> MSADSSPLVGSTPTGYGTLTIGTSIDPLSSSVSSVRLSGYCGSPWRVIGYHVVVWMMAGIPLLLFRWKPLWGVRLRLRPCNLAHAETLVIEIRDKEDSSWQLFTVQVQTEAIGEGSLEPSPQSQAEDGRSQAAVGAVPEGAWKDTAQLHKSEEAVSVGQKRVLRYYLFQGQRYIWIETQQAFYQVSLLDHGRSCDDVHRSRHGLSLQDQMVRKAIYGPNVISIPVKSYPQLLVDEALNPYYGFQAFSIALWLADHYYWYALCIFLISSISICLSLYKTRKQSQTLRDMVKLSMRVCVCRPGGEEEWVDSSELVPGDCLVLPQEGGLMPCDAALVAGECMVNESSLTGESIPVLKTALPEGLGPYCAETHRRHTLFC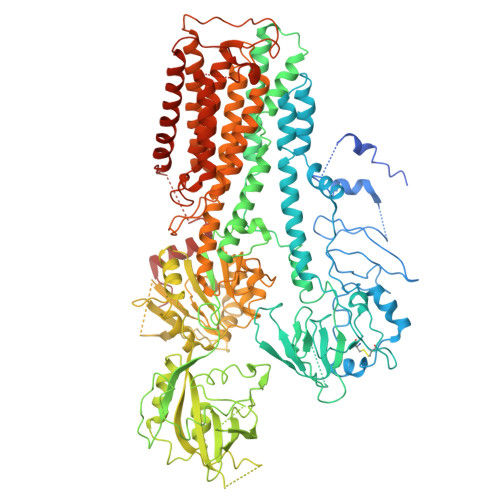GTLILQARAYVGPHVLAVVTRTGFCTAKGGLVSSILHPRPINFKFYKHSMKFVAALSVLALLGTIYSIFILYRNRVPLNEIVIRALDLVTVVVPPALPAAMTVCTLYAQSRLRRQGIFCIHPLRINLGGKLQLVCFDKTGTLTEDGLDVMGVVPLKGQAFLPLVPEPRRLPVGPLLRALATCHALSRLQDTPVGDPMDLKMVESTGPQLQAMEEPPVPVSVLHRFPFSSALQRMSVVVAWPGATQPEAYVKGSPELVAGLCNPETVPTDFAQMLQSYTAAGYRVVALASKPLPTVPSLEAAQQLTRDTVEGDLSLLGLLVMRNLLKPQTTPVIQALRRTRIRAVMVTGDNLQTAVTVARGCGMVAPQEHLIIVHATGQPASLEFLPMESPTAVNGVKDPDQAASYTVEPDPRSRHLALSGPTFGIIVKHFPKLLPKVLVQGTVFARMAPEQKTELVCELQKLQYCVGMCGDGANDCGALKAADVGISLSQAEASVVSPFTSSMASIECVPMVIREGRCSLDTSFSVFKYMALYSLTQFISVLILYTINTNLGDLQFLAIDLVITTTVAVLMSRTGPALVLGRVRPPGALLSVPVLSSLLLQMVLVTGVQLGGYFLTLAQPWFVPLNRTVAAPDNLPNYENTVVFSLSSFQYLILAAAVSKGAPFRRPLYTNVPFLVALALLSSVLVGLVLVPGLLQGPLALRNITDTGFKLLLLGLVTLNFVGAFMLESVLDQCLPACLRRLRPKRASKKRFKQLERELAEQPWPPLPAGPLR> GLVAEAEAVAAGWMLDFLCLSLCRAFRDGRSEDFRRTRNSAEAIIHGLSSLTACQLRTIYICQFLTRIAAGKTLDAQFEN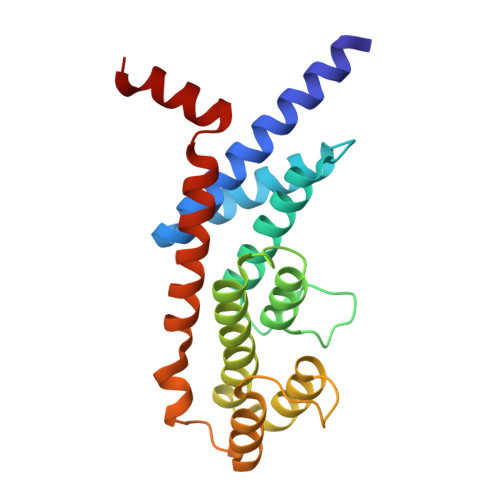DERITPLESALMIWGSIEKEHDKLHEEIQNLIKIQAIAVCMENGNFKEAEEVFERIFGDPNSHMPFKSKLLMIISQKDTFHSFFQHFSYNHMMEKIKSYVNYVLSEKSSTFLMKAAAKVVES> MGMVVALGLDFGTSGARAIACDFDSDRSVSVSVTFPKTSQNWPQVWREALWQLLTQIPADWRSRIERIAIDGTSGTVLLCDREGQPQTEPLLYNQACPIDLADLADWVPADHAALSSTSSLAKLWFWQQQFGALPPDWQILAQADWLSLQLHGCSQQSDYHNALKLGYSPDRERFSKNLLDS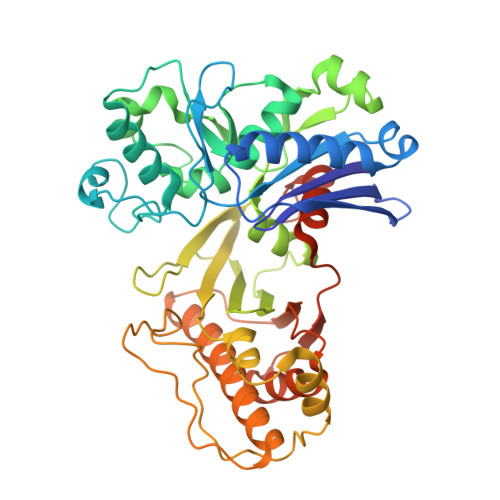ELGALLPVVHEPGVAIGPILPAIAQEFGLSPDCQICAGTTDSIAAFLASGAHQPGEAVTSLGSTIVLKLLSQVAVSDRLTGVYSHKLGGYWLTGGASNCGGATLRQFFPDTELESLSCQIDPTKKSGLDYYPLPSRGERFPIADPDRLPQLEPRPENPVQFLQGLLEGLTQVETLGYQRLQDLGATPLKRIWTAGGGAKNAVWQQLRQQAIGVPIAIAPNTEAAFGTARLAAFGLAAFHSAGLKRTLEHHHHHH> MPSLPTLQPLDLYRRTLACLVLAVSCLGGGGLWADDARTSIEQRSNAVSQVLLGIFSYVRWPKEPAVLQLSVVGPTEYADGLLRGMVQANGRRVH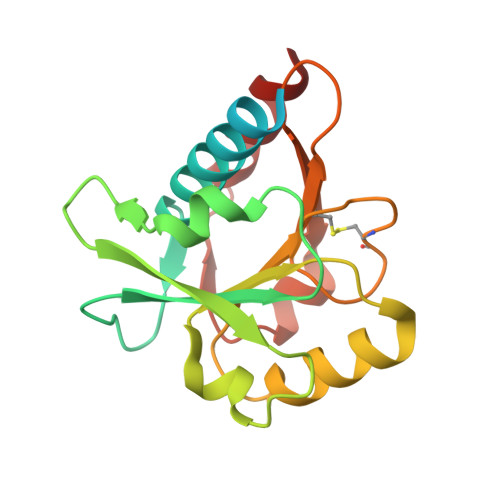AERRAVDNPDLGTLCNVIYLGVVDERERQQVFRSLAGHPVLSISERGTECSVGSMFCLNVGGPRITFEANLDSIARSGVRVHPSVLKLARRQATP>[4x]GSNRTLIVTTILEEPYVMYRKSDKPLYGNDRFEGYCLDLLKELSNILGFLYDVKLVPDGKYGAQNDKGEWNGMVKELIDHRADLAVAPLTITYVREKVIDFSKPFMTLGISILYRKGTPIDSADDLAKQTKIEYGAVRDGST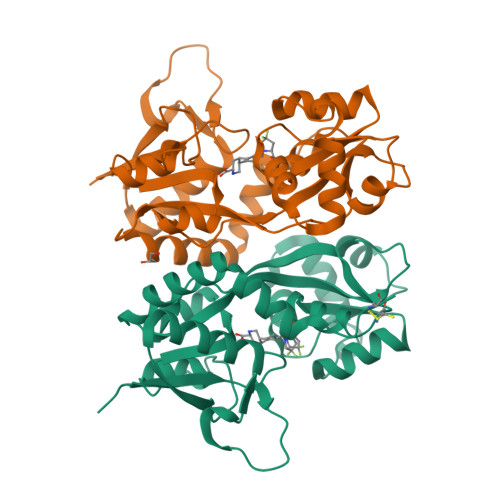MTFFKKSKISTYEKMWAFMSSRQQSALVKNSDEGIQRVLTTDYALLMESTSIEYVTQRNCNLTQIGGLIDSKGYGVGTPIGSPYRDKITIAILQLQEEGKLHMMKEKWWRGNGCPS>[2x]GSSGSSG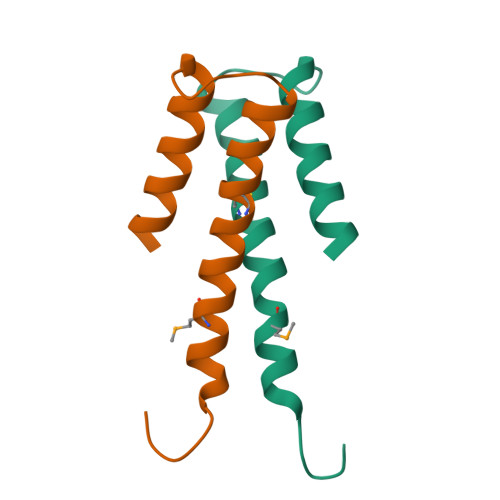GYFDAHALAMDYRSLGFRECLAEVARYLSIIEGLDASDPLRVRLVSHLNNYASQREA> MADFDNLFDAA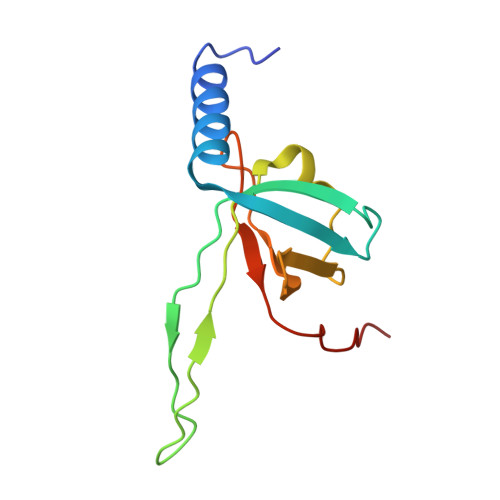IARADETIRGYMGTSATITSGEQSGAVIRGVFDDPENISYAGQGVRVEGSSPSLFVRTDEVRQLRRGDTLTIGEENFWVDRVSPDDGGSCHLWLGRGVPPAVNRRR> KLTGRDPDFHRRELWEAIEAGDFPEYEL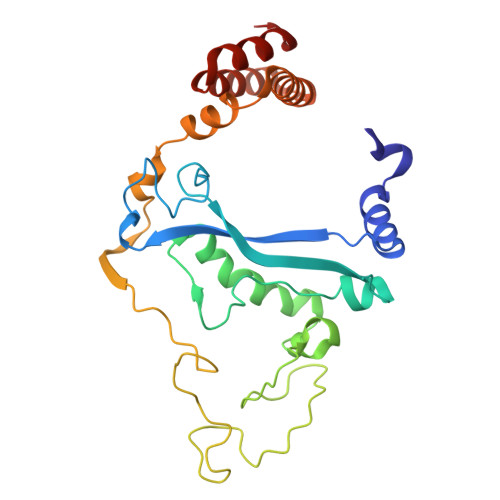GFQLIPEEDEFKFDFDLLDPTKLIPEELVPVQRVGKMVLNRNPDNFFAENEQAAFHPGHIVPGLDFTNDPLLQGRLFSYTDTQISRLGGPNFHEIPINRPTCPYHNFQRDGMHRMGIDTNPANYEPNSINDNWPRETPPGPKRGGFESYQERVEGNKVRERSPSFGEYYSHPRLFWLSQTPFEQRHIVDGFSFELSKVVRPYIRERVVDQLAHIDLTLAQAVAKNLGIELT>[6x]MTDFYTIKDAQADLAIAPLNLTVLLAPYSTTPATTLESPTDGSLAIPPGYKSVGHFEKQAGLTLGNEFDSKDIEAYGEPEPIRTIINKRTTTFDFAMYQNQRNVLELIWTQDFSNIQPSEFGGIVLEAPKVPKNIYYRAILVGMDDRNDRPIWLYWLMPKVKLDKLDNQTLNDDNVIEYKPTLKAFRDDVVGYSVAQGFAGPGWRDLVATAGFGEALTALTITPGSPTVTVATGASHTAQLLVEGDNGINYTPDVVFTSSAPDKASVSAAGLVTGVAAGSATITATKGALTATATVTVTA;>MAEFVAAQASVLIVPTLGKGANSFHQKLKEQLQTVRESVDVKIKADTAAMVAEVQATKEMLERDPINIRVETDNNGIKELVKSVTEVRHKYEDLKGDFRRGLTLNLKVVGLSALSQLGPMLASLNTSIVQLSQSSLLLPGIMSGVASSVGAAVVGSRGLTDAFKAQSDASKNVAEAGKQQRDANRAIRDSTRDLNNAIRDAKRNIEDLNAQLRDAPLDEAEAMLNLQEAQYEASQKWGKTAFQQQRDALGLAKAESQLAETRRRNVRLGQDVAEANAKGVNGNDAVVAAQERLTKALEDLAMQTGPIRALNDAMAKLSPNARDFVDQVSSLKGAWDGLRSTVQDRLFDGLGASVQTLAGQDLPILERGLAGIAGAINGNLKTAMSQLATDENKGFLGRIFGNTEEAQNRFSTALKPLLDSFMQLSAVGSDYLPRLSNAFGDVLNRFDGFIERADADGSLDKWINNGLDAMTQLGNSLINVGSIMNTISEAFTGTGGKGLLELLETGTKRLADFLKGAEGQQKLKQFFLDARTELNNWKPLLSQLPGLIKNVATAGQQWANLVLPFLTSAASLLKEHPGLVTAIFTAYMTWRTISPIIGTINLLLSSETGMVGAAKKAGRAVGKGEGLTGKLGVLAGMVGQGGVVMTGLSLVAGFLINEWVTAQNEAAEAVSYHASMISRLKGEMDGLTGSLTTQGLQGKLDAARQWTDIHQTDGKPKDLVAAANSFGVDLPTFMGALTPTNQAARNAVTGKARQTVLDDLNKQGLETVLGKDALNALNLYNQNAAPDKKITNDVLADIATGVNPESKKLFEDAKKSNLIHFNESDLLYGYNKPWGFIPGTDPSGKGLSPVARDAANVSGFVLNDTGNALQVGSDIRSTNEALYGKAVLTPAGQQMFGQFGSPQASFENGSKDAAVRVDTTLQNLPPQFVKDVESNGGHFEELPDGVIIHMRKDRAAQYVTAGSYAGGGFLSGPGTGRSDSMLARVSNGEFITRAASVAKYGRGLFDALNSGTLDPSMLPRFDSGGLVDIFLPGGGTAAPPPTGSANPVDLARGLPRGPAVQSAPANRFDPSPLPTDLLPKPVIPMPDLANPGLYDPATGKYGAAPASAVQQPLKPGVDGDKGETSGPNVPPTDPRSPGYKQPNHGLGGSPGPGNGTPHLTGPGGTPVSPGAASALPSNGGIPGLTPSATDPLGLSGLPKEIQPVTILEQIGEILLSAVLGFFGLDPTYFNIGKRIFTGIKGDKPNEANPGVQSILDGYKNPLADGQNPYVGTSIYDASFDPASQRASNMAELMRGKPYTWGGSSLDGTDCSGLVMYVVDAYEGKEFSGRTGGTGGFASSLPAKGGVIISDPSQAPPGTLRVGWNASHTAGTLPDGRNFESSTFGKPIAVGAGASGYNDPQFTNWAYFPAPGYANGGFLSGAGTGRSDSMLARVSNGEFITRASSVAKYGRSLFDALNAGTVDPGMLPGFADGTPPIPGLPVPQPQTPQQAGPLPDPNGQDAQAAQQVTDTAASALDGVAGAMNGVNMGSSGAIPGADAPDGAQQGKDPRSILGAAPTNTDHNNPALSKGIQGAFSTVGSLASMAASAAMSAGTMGAGAAGASGAAGSGIQAGAQIAGQVATGALNILSSLLVGSAPGSTGTTQSAYGAPVLPQGPPQSSGGGPAVVNNYGDIHTANYDEFYKGQQRREAQQQAPILPVR[3x];>MLSTGPIMETLTLTVGSAFEIPGWKLRGEYPAGTTSHLVFTDAAGGTLGEFEGTVSAKEIHYLQAPDDVKNIPHGANFQLFVTYPSMQPQCLYFGTAIRKEPRYPLSTVVSPEDSAVQYKANFVGQYIGPMWKPMGNGWGSLGIHTHALISEAPSMGPNYSLFSSAAARWLWSMNMDSVTIVVRVLNVGAGKFNVIVCADYQMQTYLGIQFETGISNNKVHVITGDGPLNWGYQGDAVNNTTANGDVYTIKYNDLLDTISCYKGTSLTPLIEASGLDVPHGEGFRYTGLAWNTALLSPGVEPTAWEAKDGV[12x];>MTDFLKIELIGRDGSHWVLSGPGMGQQGVTLNPNLQQFYDAPVKTLYVPGPFGEEYAGKRVQRREIVFSVQAYDEDPDTWSTVDSLWRWAWDYDEESELRVSTSDGTRFLKVRLMEEPKPYYEKDPHITADNPIVMTVTATFPYWQDEPEELIWTTLSTEDMTRFPVRNDGDVPVWLKWTLTAPGLWILPDFSWGNDMYSRGREDLGRTVAMPELVAGEHVSVDSDPRVQTLIAVNGMPTQNRWKGNDLLYPLMPGKGAEIPVQLKNAPEGGACKLTRPRWYSRPWSRPGVRLNG[6x];>[3x]MANNWTDILAASDGDEWAAFKTIEAQADEVRAGHQALRRAKPLIRLWMNNPDGSEGLVYVGRVDYDDTIRGSFPFKNNTPSQGVLELRDDNYLAVWLKQLPNNPELKKNVVITVDFYGGKKRWSGLLDKWTIKSKEHVKYLEVTFNDDLTMLQYLLCPPNPALPIPVLQFPRIFGIAGPAKWAISTLIFINLFRVQGNLWTLPDDPFNLESWDDILDWSDWQCFVKSNSFLLDDSSVWTFLSSRMNPVDSIIADALDDAQLTITYRRVLTDDGETAEGFPGAHGIKNGALVFEIVDNSNATALEGTFFSGTIVDGFARSVLLYGGGFVEDTLSVVSDDQTLQPDEYYQSGWLATMAKMPWLVVRDNEWTPIESSDLSWGPAKNVSVIVGGDNPAADAIAKLIIETTGNLLGYFLLGGFSSAGTIAADIIMPFLVGTIAAWLQWKNTGRATELGWVHYWELYQQGAETNSWSLAALAALRGGFLVGRSETVHLMALHDSWIIPGLHIDIGQRMGSTVNSKGVENIVWVNQLEEMTAAWDNSAGQTMPLSWVLKAGKSDRAMSIGERVARLAKKMSEALNNVGVHIVQS;>[3x]MTMPNGSGGLDPGAWLSHWVNQADLSSLAGRTEDEVRAYFENLVQADSGWGDASNTFFNLILGGFQNLSEFVTLIVQAVTGAPGGLTDLQAFLTERWGDLADAFQAVANLIDAIAGEVGSSLADAIAKLATFLTELSPLNAGMLFGLIGTNHLPLLSVSHIANINPELLVNAGFDSDVSVVDNPYWDWDGTVGRTAPLGAVKVVADGTIKDLLSGPDAIPVVEGQKLNVSAWLKYSGLVAGAGAGSIRLSGTAYSADGEVVAY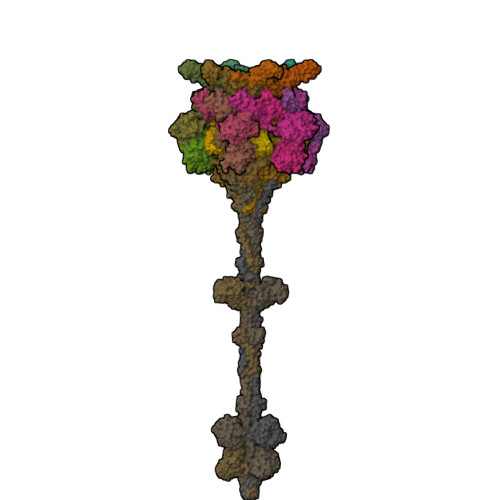PDFGGIPDGASGTSDWTQVTGQYVVPAGVTQFRLRLSVRENATGGTVWFDDCSVKKAGLLPQGLVDGLVQALSDLLTWLESLVDNVLSALGLDPIGTIVDKILDLADEFGDWLGATEDTAANLSNLLTKLLSDPASVIGPLAQSMITGLTGALGNLNTAINQIGDVLVGTVVTPINSAISNVIDWFNSLLNFQDTTTSNQINQQNFQIATLASGIKKQQWECRYSTAFVTFPEMFCDWGFALGGTTGAQSTGTAHTHTLNTDGLAALQIQILPAGYAIGGYIGISDTTIVDTIAMKMYKETSSAINNVYLEVFREDSTGALTSVGSVDVSGQLTTASDYVEATLPAGVIVNAGERYVVRMRNATTVGNRVGVSVMKELVGGRELSIRTETATDSNKTFYTPSEVLTAQGVSVIMPWAMMAAKNLATTDQSFSDDFNRSAMGGLWFLKSDTGTNQVGVSGGRAAFSGLTDGNQNALYIRPTAGDKQWVEATLYETGIAASGAREGLLMHANRDLSQVVYLGVNLNTAKIYTGPWNSLTERASVSTTGNDVLWQMYFDPATAAYTVLKNGQASGLTWTDSGSVVAHGPNYRFGGLRISRATFFNAGRIDNWTLKDWA> MSNISRQAYADMFGPTVGDKVRLADTELWIEVEDDLTTYGEEVKFGGGKVIRDGMGQGQMLAADCVDLVLTNALIVDHWGIVKADIGVKDGRIFAIGKAGNPDIQPNVTIPIGAATEVIAAEGKIVTAGGIDTHIHWICPQQAEEALVSGVTTMVGGGTGPAAGTHATTCTPGPWYISRMLQAADSLPVNIGLLGKGNVSQPDALREQVAAGVIGLKIHEDWGATPAAIDCALTVADEMDIQVALHSDTLNESGFVEDTLAAIGGRTIHTFHTEGAGGGHAPDIITACAHPNILPSSTNPTLPYTLNTIDEHLDMLMVC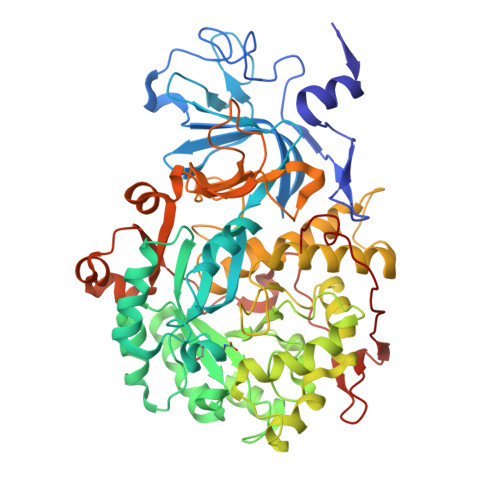HHLDPDIAEDVAFAESRIRRETIAAEDVLHDLGAFSLTSSDSQAMGRVGEVILRTWQVAHRMKVQRGALAEETGDNDNFRVKRYIAKYTINPALTHGIAHEVGSIEVGKLADLVVWSPAFFGVKPATVIKGGMIAIAPMGDINASIPTPQPVHYRPMFGALGSARHHCRLTFLSQAAAANGVAERLNLRSAIAVVKGCRTVQKADMVHNSLQPNITVDAQTYEVRVDGELITSEPADVLPMAQRYFLF(3~{S})-3-[(1~{S},3~{a}~{S},4~{E},7~{a}~{S})-7~{a}-methyl-4-[(2~{Z})-2-[(5~{S})-2-methylidene-5-oxidanyl-cyclohexylidene]ethylidene]-2,3,3~{a},5,6,7-hexahydro-1~{H}-inden-1-yl]-3-oxidanyl-~{N}-propan-2-yl-butanamide 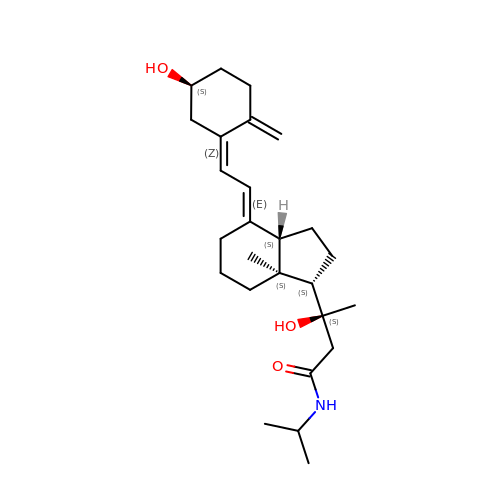| C26 H41 N O3 | CSLRSUXCVDRFJS-YDGCZWIRSA-N>[4x]MSYTVGTYLAERLVQIGLKHHFAVAGDYNLVLLDNLLLNKNMEQVYCCNELNCGFSAEGYARAKGAAAAVVTYSVGALSAFDAIGGAYAENLPVILISGAPNNNDHAAGHVLHHALGKTDYHYQLEMAKNITAAAEAIYT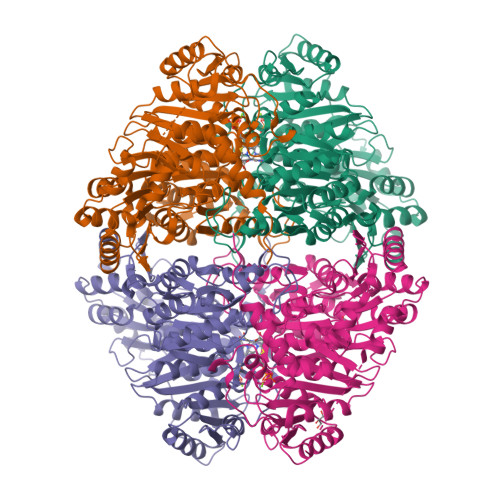PEEAPAKIDHVIKTALREKKPVYLEIACNIASMPCAAPGPASALFNDEASDEASLNAAVEETLKFIANRDKVAVLVGSKLRAAGAEEAAVKFADALGGAVATMAAAKSFFPEENPHYIGTSWGEVSYPGVEKTMKEADAVIALAPVFNDYSTTGWTDIPDPKKLVLAEPRSVVVNGIRFPSVHLKDYLTRLAQKVSKKTGALDFFKSLNAGELKKAAPADPSAPLVNAEIARQVEALLTPNTTVIAETGDSWFNAQRMKLPNGARVEYEMQWGHIGWSVPAAFGYAVGAPERRNILMVGDGSFQLTAQEVAQMVRLKLPVIIFLINNYGYTIDVMIHDGPYNNIKNWDYAGLMEVFNGNGGYDSGAGKGLKAKTGGELAEAIKVALANTDGPTLIECFIGREDCTEELVKWGKRVAAANSRKPVNKLL> MGKYLLPTAAAGLLLLAAQPAMDFTIQDIRVEGLQRTEPSTVFNYLPVKVGDTYNDTHGSAIIKSLYATGFFDDVRVETADGQLLLTVIERPTIGSLNITGAKMLQNDAIKKNLESFGLAQSQYFNQATLNQAVAGLKEEYLGRGKLNIQITPKVTKLARNRVDIDITIDEGKSAKITDIEFEGNQVYSDRKLMRQMSLTEGGIWTWLTRSDRFDRQKFAQDMEKVTDFYQNNGYFDFRILDTDIQTNEDKTRQTIKITVHEGGRFRW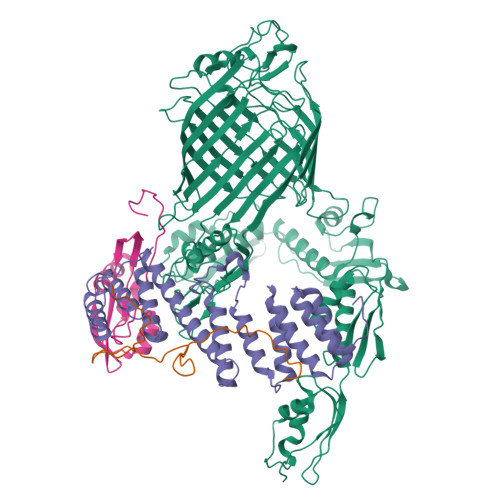GKVSIEGDTNEVPKAELEKLLTMKPGKWYERQQMTAVLGEIQNRMGSAGYAYSEISVQPLPNAGTKTVDFVLHIEPGRKIYVNEIHITGNNKTRDEVVRRELRQMESAPYDTSKLQRSKERVELLGYFDNVQFDAVPLAGTPDKVDLNMSLTERSTGSLDLSAGWVQDTGLVMSAGVSQDNLFGTGKSAALRASRSKTTLNGSLSFTDPYFTADGVSLGYDIYGKAFDPRKASTSVKQYKTTTAGGGVRMGIPVTEYDRVNFGLAAEHLTVNTYNKAPKRYADFIRKYGKTDGADGSFKGLLYKGTVGWGRNKTDSASWPTRGYLTGVNAEIALPGSKLQYYSATHNQTWFFPLSKTFTLMLGGEVGIAGGYGRTKEIPFFENFYGGGLGSVRGYESGTLGPKVYDEYGEKISYGGNKKANVSAELLFPMPGAKDARTVRLSLFADAGSVWDGRTYTAAENGNNKSVYSENAHKSTFTNELRYSAGGAVTWLSPLGPMKFSYAYPLKKKPEDEIQRFQFQLGTTF;> MGQLRKLLLPGLLSVTLLSGCGMGSGSKTEQPKLDYQSRSHRLIKLEVPPDLNNPDQGNLYRLPAGSGAVRASDLEKRRTPAVQQPADAEVLKSVKGVRLERDGSQRWLVVDGKSPAEIWPLLKAFWQENGFDIESEEPAIGQMETEWAENRAKIPQDSLRRLFDTVGLGGIYSTGERDKFIVRIEQGKNGVSDIFFAHKAMKEVYGDKNKDTTMWQPSASDPNLEAAFLTRFMQYLGVDGRQAENALAKKPTLPAANEMARIEGKSLIVFGDYGRNWRRTGLALDRIGLTVVGQNTERHAFLVQKAPNESNAVTEQKPGLFKRLLGKGKAEKPAEQPELIVYAEPVADGSRIVLLNKDGSAYAGKDASALLGKLHSELR;> MQLRKLLLPGLLSVTLLSGCAMGATQGTADKDAQITQDWSVEKLYAEAQDELNSSNYTRAVKLYEILESRFPTSRHARQSQLDTAYAYYKDDEKDKALAAIERFRRLHPQHPNMDYALYLRGLVLFNEDQSFLNKLASQDWSDRDPKANREAYQAFAELVQRFPNSKYAADATARMVKLVDALGGNEMSVARYYMKRGAYIAAANRAKKIIGSYQNTRYVEESLAILELAYKKLDKPQLAADTRRVLETNFPKSPFLTHAWQPDDMPWWRYWH;> MQLRKLLLPGLLSVTLLSGCAMDSVERVSLFPSYKLKIIQGNELEPRAVAALRPGMTKDQVLLLLGSPILRDAFHTDRWDYTFNTSRNGIIKERSNLTVYFENGVLVRTEGDALQNAAEALRAKQNADKQHHHHHHHHHH[[(2~{R},3~{S},4~{R},5~{R})-5-(2-azanyl-6-oxidanylidene-1~{H}-purin-9-yl)-3,4-bis(oxidanyl)oxolan-2-yl]methoxy-oxidanyl-phosphoryl] [(2~{R},3~{S},4~{R},5~{S},6~{R})-5-fluoranyl-6-(hydroxymethyl)-3,4-bis(oxidanyl)oxan-2-yl] 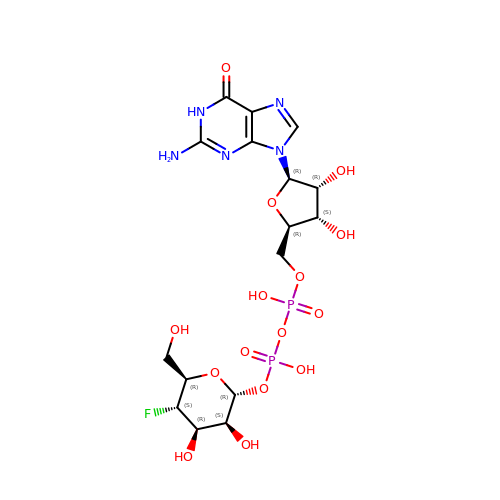hydrogen phosphate | C16 H24 F N5 O15 P2 | LDMYSLGOFVDHNN-YVXBHLEUSA-N>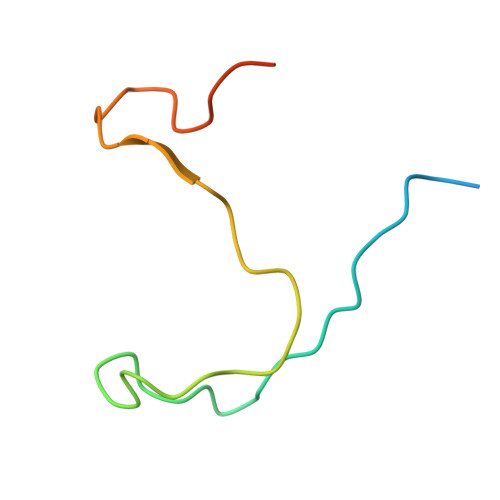 GSRMLPIEGAPRRRPPVKFIFPPPPLSSLPGFGRPRGYAGPTVIDMSAPDDVFAEDTPSPPAT>[12x]MNRDTSPDLHYLSGFGNEFASEALPGALPVGQNSPQKAPYGLYAELLSGTAFTMARSELRRTWLYRIRPSALHPRFERLARQPLGGPLGGINPNRLRWSPQPIPAEPTDFIEGWLPMAANAGAEKPAGVSIYIYRAN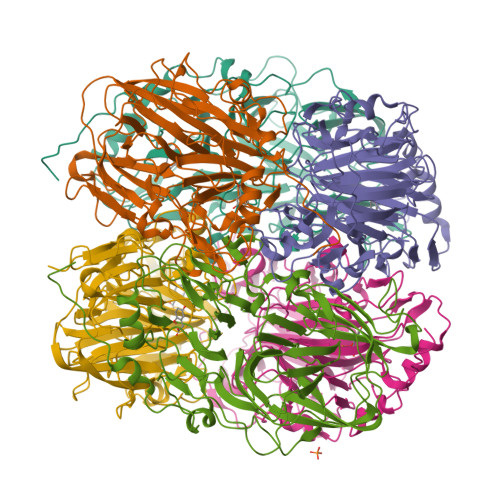RSMERVFFNADGELLLVPEQGRLRIATELGVMEVEPLEIAVIPRGMKFRVELLDGQARGYIAENHGAPLRLPDLGPIGSNGLANPRDFLTPVAHYEEAEGPVQLVQKFLGEHWACELQHSPLDVVAWHGSNVPYKYDLRRFNTIGTVSFDHPDPSIFTVLTSPTSVHGMANMDFVIFPPRWMVAENTFRPPWFHRNLMNEFMGLINGAYDAKAEGFLPGGASLHGVMSAHGPDAETCEKAIAADLAPHKIDNTMAFMFETSQVLRPSLQALECPQLQADYDSCWATLPSTFNPNRR> GPHM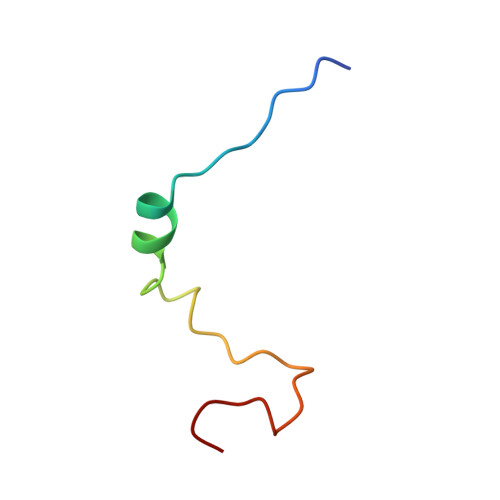TKLIYERAFMKNLRGSPLSQTPPSNVPSCLLRGT> NGDRLYRADSRPPDEIKRSGGLMPRGHNEYFDRGTQMNINLYDHARGTQTGFVRYDDGYVSTSLSLRSAHLAGQSILSGYSTYYIYVIATAPNMFNVNDVLGVYSPHPYEQEVSALGGIPYSQIYGWYRVNFGVIDERLHRNREYRDRYYRNLNIAPAEDGYRLAGFPPDHQAWREEPWIHHAPQGCGNSSR;> TITGDTCNEETQNLSTIYLREYQSKVKRQIFSDYQSEVDIYNRIRDEL;>APQTITELCSEYRN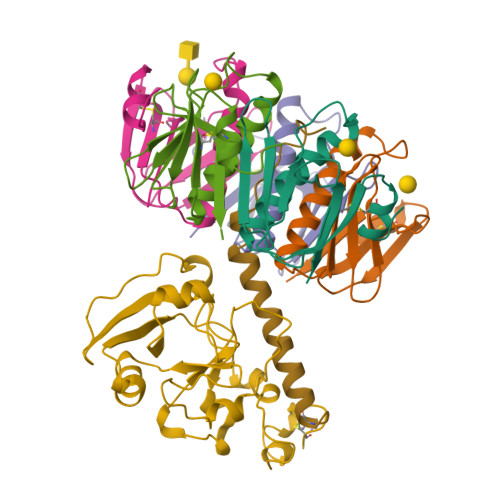TQIYTINDKILSYTESMAGKREMVIITFKSGETFQVEVPGSQHIDSQKKAIERMKDTLRITYLTETKIDKLCVWNNKTPNSIAAISMKN[5x]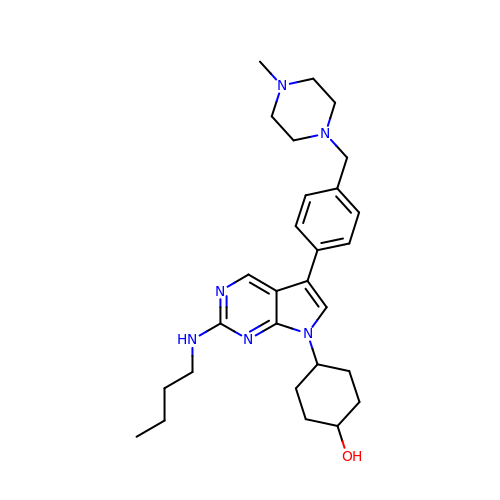4-[2-(butylamino)-5-[4-[(4-methylpiperazin-1-yl)methyl]phenyl]pyrrolo[2,3-d]pyrimidin-7-yl]cyclohexan-1-ol | C28 H40 N6 O | MJSHVHLADKXCML-RQNOJGIXSA-N> MEVTHKQFDLSGFLPDQAPDTLKSGAISRGFNVKPTILGWEKSGGFRETNTAPTNEKDFIFFWSPAIGDNRWFSGGDKTVQQVEGNVVSDVSRTGGYTAGSGRRWNAVNFNGVLLMNNELDSPQYLAASGKLEDFPNLPSNVRFRTVAVYKNFILGLGVNFGSGFLDDEIYWSHQADPGTMPPNWDYANAASDSGRTPLPSEGYCVTSEELGSMNIVYKSDSIWTMQLIGGQWIFRFENKFPGQGILNKKSVVSFEGKHFVVTQKDIIVHDGYQVRSVADKRVRNFFFTDMNSDYFERVFVVKDPRVAEVYVFYPSKNSVDGLCDRALVWNWRDDVWSLLNLRPLKHAAYGYEITGV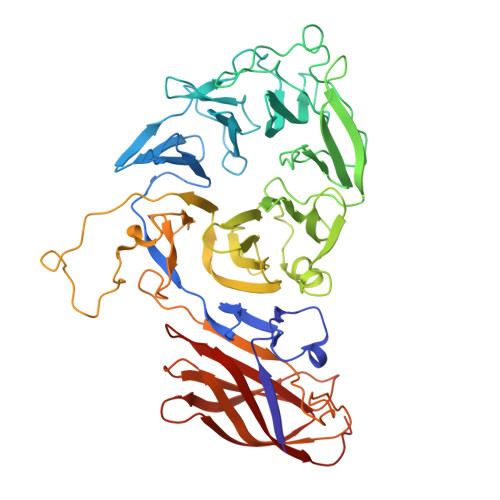SITWDNFVGGWESTGLWQADEDVAKYAPVLHYSFRDVPKLLAPTPQALFIDEEIEAVWEREDIVIGSISRDGVPYQDYERNKSVSSISFDVDTTEPFDVYIGYKGSLEDSVEWEFAGTVNPMEDKRLFCLLTAGLFSMRIISKAQTFILRSYKITYEFAGEMWS> MAHHHHHHMEQNYLYKGTTTLK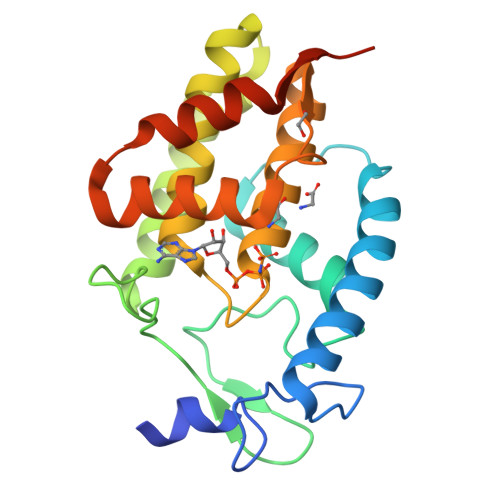NKYGIKDPNKLYERCNHDVVKEAVNFRHEPPPQNFDAAYLSLIHWSLFHKTFEWAGHTRDTSFTFEDGTTARMPAMRPKGYEAPFAIGPQIKKELKQLEKTLNQKNNLKGLSHQEFAENAADVFMALEHAHPFRKGNGRANRMFMEKLGQAAGHTVDFSFITKGRMTTACIEAMQYGNSQPMKDLFEDITHPQKSVILKEFISQM>[2x]MVEHDKSGSKRQELRSNMRNLITLNKGKFKPTASTAEGDEDDLSFTLLDSVFDTLSDSITCVLGSTDIGAIEVQQFMKDGSRNVLASFNIQTFDDKLLSFVHFADINQLVFVFEQGDIITATYDPVSLDPAETLIEIMGTIDNGIAAAQWSYDEETLAMVTKDRNVVVLSKLFEPISEYHLEVDDLKISKHVTVGWGKKETQFRGKGARAMEREALASLKASGLVGNQLRDPTMPYMVDTGDVTALDSHEITISWRGDCDYFAVSSVEEVPDEDDETKSIKRRAFRVFSREGQLDSASEPVTGMEHQLSWKPQGSLIASIQRKTDLGEEDSVDVIFFERNGLRHGEFDTRLPLDEKVESVCWNSNSEALAVVLANRIQLWTSKNYHWYLKQELYASDISYVKWHPEKDFTLMFSDAGFINIVDFAYKMAQGPTLEPFDNGTSLVVDGRTVNITPLALANVPPPMYYRDFETPGNVLDVACSFSNEIYAAINKDVLIFAAVPSIEEMKKGKHPSIVCEFPKSEFTSEVDSLRQVAFINDSIVGVLLDTDNLSRIALLDIQDITQPTLITIVEVYDKIVLLRSDFDYNHLVYETRDGTVCQLDAEGQLMEITKFPQLVRDFRVKRVHNTSAEDDDNWSAESSELVAFGITNNGKLFANQVLLASAVTSLEITDSFLLFTTAQHNLQFVHLNSTDFKPLPLVEEGVEDERVRAIERGSILVSVIPSKSSVVLQATRGNLETIYPRIMVLAEVRKNIMAKRYKEAFIVCRTHRINLDILHDYAPELFIENLEVFINQIGRVDYLNLFISCLSEDDVTKTKYK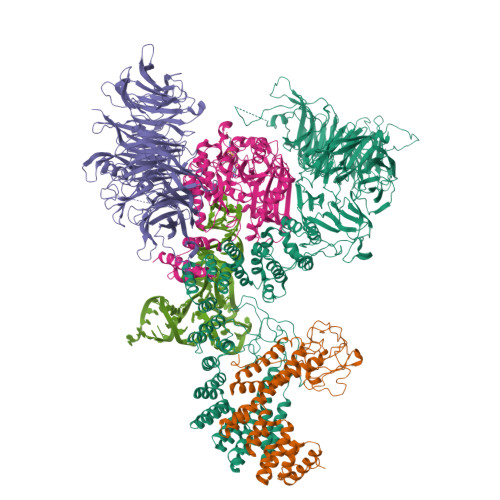ETLYSGISKSFGMEPAPLTEMQIYMKKKMFDPKTSKVNKICDAVLNVLLSNPEYKKKYLQTIITAYASQNPQNLSAALKLISELENSEEKDSCVTYLCFLQDVNVVYKSALSLYDVSLALLVAQKSQMDPREYLPFLQELQDNEPLRRKFLIDDYLGNYEKALEHLSEIDKDGNVSEEVIDYVESHDLYKHGLALYRYDSEKQNVIYNIYAKHLSSNQMYTDAAVAYEMLGKLKEAMGAYQSAKRWREAMSIAVQKFPEEVESVAEELISSLTFEHRYVDAADIQLEYLDNVKEAVALYCKAYRYDIASLVAIKAKKDELLEEVVDPGLGEGFGIIAELLADCKGQINSQLRRLRELRAKKEENPYAFYGQETEQADDVSVAPSETSTQESFFTRYTGKTGGTAKTGASRRTAKNKRREERKRARGKKGTIYEEEYLVQSVGRLIERLNQTKPDAVRVVEGLCRRNMREQAHQIQKNFVEVLDLLKANVKEIYSISEKDRERVNENGEVYYIPEIPVPEIHDFPKSHIVDF;> MVECITPEAIFIGANKQTQVSDIHKVKKIVAFGAGKTIALWDPIEPNNKGVYATLKGHEAEVTCVRFVPDSDFMVSASEDHHVKIWKFTDYSHLQCIQTIQHYSKTIVALSALPSLISVGCADGTISIWRQNIQNDEFGLAHEFTIKKGFFYPLCLSLSKVEEKKYLLAIGGTNVNVFIASFILSDSGIEKCRVVAELEGHEDWVKSLAFRHQETPGDYLLCSGSQDRYIRLWRIRINDLIDDSEEDSKKLTLLSNKQYKFQIDDELRVGINFEALIMGHDDWISSLQWHESRLQLLAATADTSLMVWEPDETSGIWVCSLRLGEMSSKGASTATGSSGGFWSCLWFTHERMDFFLTNGKTGSWRMWATKDNIICDQRLGISGATKDVTDIAWSPSGEYLLATSLDQTTRLFAPWIYDASGRKREIATWHEFSRPQIHGYDMICVETVTDTRFVSGGDEKILRSFDLPKGVAGMLQKFVGIQFEEKSEMPDSATVPVLGLSNKAGEDDANEDDEEEEGGNKETPDITDPLSLLECPPMEDQLQRHLLWPEVEKLYGHGFEITCLDISPDQKLIASACRSNNVQNAVIRIFSTENWLEIKPALPFHSLTITRLKFSKDGKFLLSVCRDRKWALWERNMEDNTFELRFKNEKPHTRIIWDADWAPLEFGNVFVTASRDKTVKVWRHQKEPADDYVLEASIKHTKAVTAISIHDSMIREKILISVGLENGEIYLYSYTLGKFELITQLNEDITPADKITRLRWSHLKRNGKLFLGVGSSDLSTRIYSLAYE;> MARHGKGPKTNKKKLAPEKERFIQCCADITLELTDSLTSGTTREINLNGLITKYSKKYKLKQQPRLTDIINSIPDQYKKYLLPKLKAKPVRTASGIAVVAVMCKPHRCPHIAYTGNICVYCPGGPDSDFEYSTQSYTGYEPTSMRAIRARYDPYEQARGRVEQLKQLGHSIDKVEYVLMGGTFMSLPKEYREDFIVKLHNALSGFNGNDIDEAILYSQQSLTKCVGITIETRPDYCTQTHLDDMLKYGCTRLEIGVQSLYEDVARDTNRGHTVRSVCETFAVSKDAGYKVVSHMMPDLPNVGMERDIEQFKEYFENPDFRTDGLKIYPTLVIRGTGLYELWKTGRYKSYSANALVDLVARILALVPPWTRIYRVQRDIPMPLVTSGVDNGNLRELALARMKDLGTTCRDVRTREVGIQEVHHKVQPDQVELIRRDYYANGGWETFLSYEDPKKDILIGLLRLRKASKKYTYRKEFTSQRTSIVRELHVYGSVVPLHSRDPRKFQHQGFGTLLMEEAERIAKEEHGSEKISVISGVGVRNYYGKLGYELDGPYMSKRI>MGNRLSKIATRTGDDGTTGLGDGSRVRKDDARIAAIGDVDELNSQIGVLLAEPLPDDVRAALSAIQHDLFDLGGELCIPGHAAITDAHLARLDGWLAHYNGQLPPLEEFILPGGARGAALAHVCRTVCRRAERSIVALGA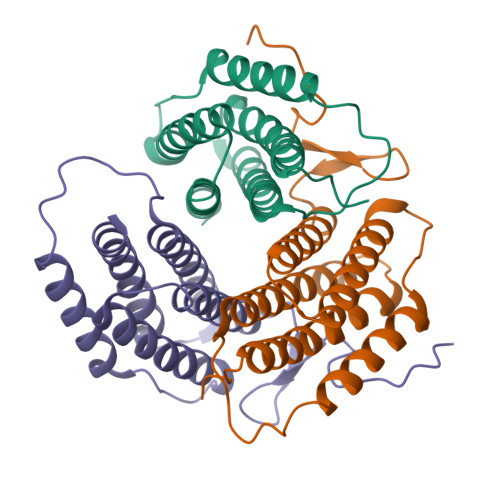SEPLNAAPRRYVNRLSDLLFVLARVLNRAAGGADVLWDRTRAH[3x]>[4x]GAMGSMSDSSPTINFINFNQTGTCISLGTSKGFKIFNCEPFGKFYSEDSGGYAIVEMLFSTSLLALVGIGDQPALSPRRLRIINTKKHSIICEVTFPTSILS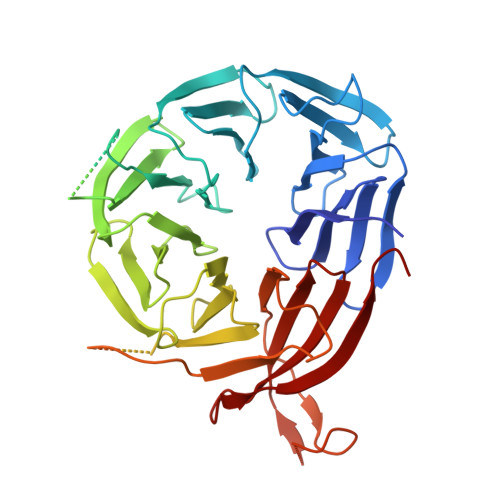VKMNKSRLVVLLQEQIYIYDINTMRLLHTIETNPNPRGLMAMSPSVANSYLVYPSPPKVINSEIKAHATTNNITLSVGGNTETSFKRDQQDAGHSDISDLDQYSSFTKRDDADPTSSNGGNSSIIKNGDVIVFNLETLQPTMVIEAHKGEIAAMAISFDGTLMATASDKGTIIRVFDIETGDKIYQFRRGTYATRIYSISFSEDSQYLAVTGSSKTVHIFKLGHSMSNNKLDSDDSNMEEAAADDSSLDTTSIDALSDEENPTRLAREPYVDASRKTMGRMIRYSSQKLSRRAARTLGQIFPIKVTSLLESSRHFASLKLPVETNSHVMTISSIGSPIDIDTSEYPELFETGNSASTESYHEPVMKMVPIRVVSSDGYLYNFVMDPERGGDCLILSQYSILMD>[6x]GSMTLVIKTNEDLNKLNDNIHTLTIGANFNQPIEHIKWPKLLTTLTFEWYFDQPIENVKLPDSLTTLTFGYSFNQPIEKVKWPKTLAFLTFGYKFNKPIEKVKWPDSLTTLIFEENSLFDQSIEKIKWSNSLTTLIFGWNFNQPIENVEWPESLTTLVFNEDSIFNQPIENVKWPKLLKTIIFGCHFNHPIENVKWPGSLTTLIFGDDFNQP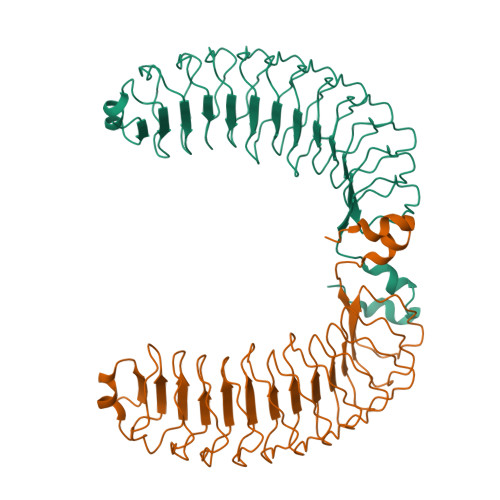FENVILPKSLTNLTFGPNFNQPLNFLPESLKNITITTNYQQNLYNLPSSLNCIKIISYKRTYEHIVNVLPEHLKKKVIKI> MKEKLVAIVGPTAVGKTKTSVMLAKRLNGEVISGDSMQVYRGMDIGTAKITAEEMDGVPHHLIDIKDPSESFSVADFQDLATPLITEIHERGRLPFLVGGTGLYVNAVIHQFNLGDIRADEDYRHELEAFVNSYGVQALHDKLSKIDPKAAAAIHPNNYRRVIRALEIIKLTGKTVTEQARHEEETPSPYNL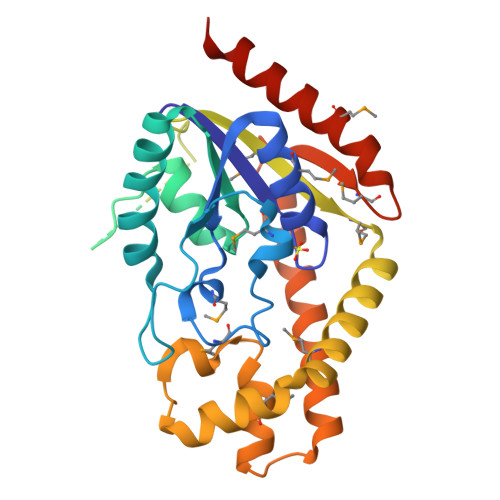VMIGLTMERDVLYDRINRRVDQMVEEGLIDEAKKLYDRGIRDCQSVQAIGYKEMYDYLDGNVTLEEAIDTLKRNSRRYAKRQLTWFRNKANVTWFDMTDVDFDKKIMEIHNFIAGKLEEKSKLEHHHHHH THIENO[3,2-B]PYRIDINE-2-SULFONIC ACID [2-OXO-1-(1H-PYRROLO[2,3-C]PYRIDIN-2-YLMETHYL)-PYRROLIDIN-3-YL]-AMIDE 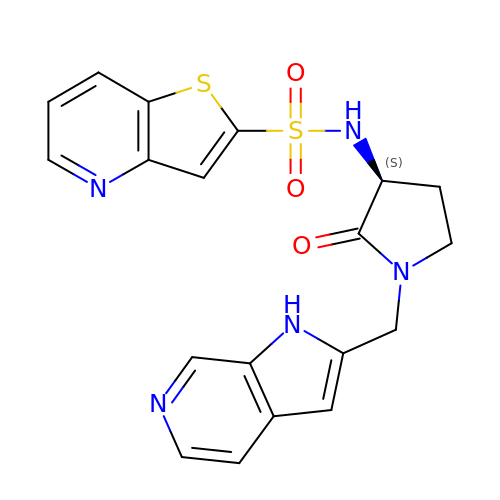| C19 H17 N5 O3 S2 | PLXOQMHGHDZMSX-AWEZNQCLSA-N> MQYLLPEAKAQD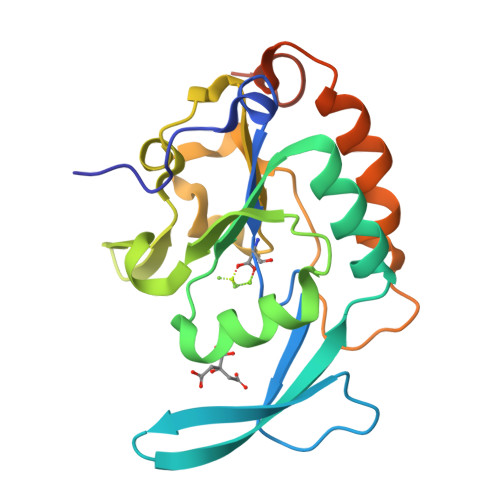SDKICVVIDLDETLVHSSFKPVNNADFIIPVEIDGVVHQVYVLKRPHVDEFLQRMGELFECVLFTASLAKYADPVADLLDKWGAFRARLFRESCVFHRGNYVKDLSRLGRDLRRVLILDNSPASYVFHPDNAVPVASWFDNMSDTELHDLLPFFEQLSRVDDVYSVLRQPRPGSAAALEHHHHHH> SMPSQMEHAMETMMFTFHKFAGDKGYLTKEDLRVLMEKEFPGFLENQ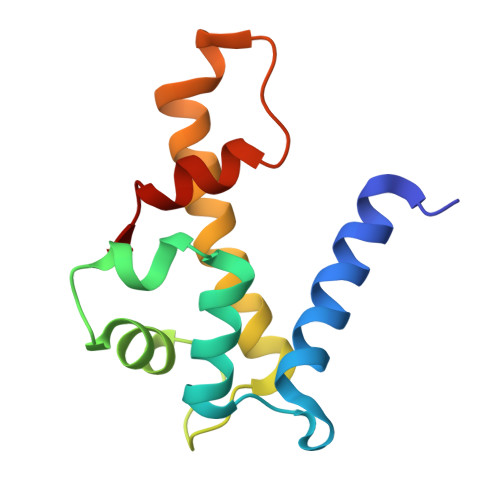KDPLAVDKIMKDLDQCRDGKVGFQSFFSLIAGLTIACNDYFVVHMKQENLYFQGDSTVHEILSKLSLE> MATRPTSVEMEPIDDSHHLDKILLQARELSQPI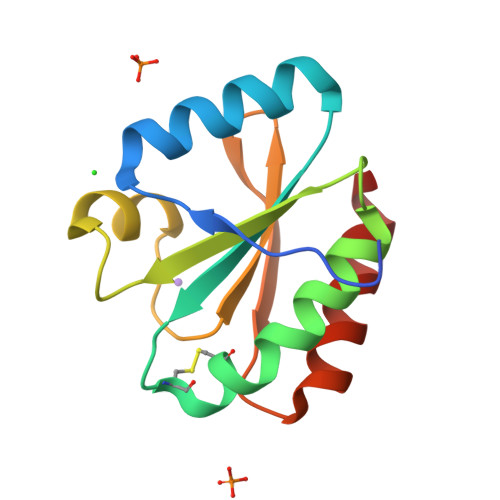IIDWMASWCRKCIYLKPKLEKLAAEYDTKIKFYCADVNKVPQALVKRGNISKMPTIQLWKDGEMKAEVIGGHKAWLVIEEVREMIQKFV> MVVSENVVSAPMPGKVLRVLVRVGDRVRVGQGLLVLEAMKMENEIPSPRDGVVKRILVKEGEAVD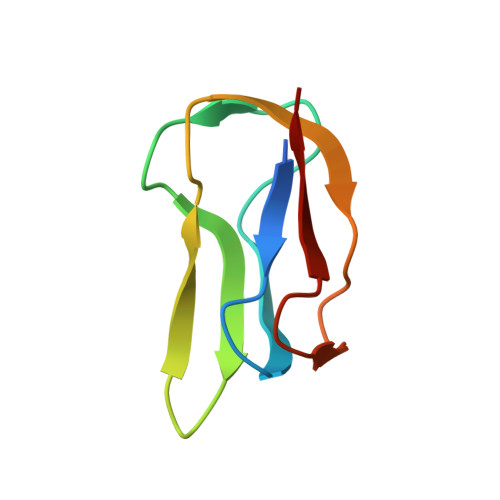TGQPLIELG>MAAQNEQRPERIKTTPYLEGDVLSSDSGPLLSVFALQEIMQKVRQVQADYMTATREVDFTVPDVQKILDDIKALAAEQVYKIVKVPSISFRHIVMQSRDRVLRVDTYYEEMSQVGDVITEDEPEKFYSTIIKKVRFIRGKGSFILHDIPTRDHRGMEVAEPEVLGVEFKNVLPVLTAEHRAMIQNALDGSIIENGNVATRDVDVFIGACSEPVYRIYNRLQGYIEAVQLQELRNSIGWLERLGHRKRITYSQEVLTDFRRQDTIWVLALQLPVNPQVVWDVPRSSIANLIMNIATCLPTGEYIAPNPRISSITLTQRITTTGPFAILTGSTPTAQQLNDVRKIYLALMFPGQIILDLKIDPGERMDPAVRMVAGVVGHLLFTAGGRFTNLTQNMARQLDIALNDYLLYMYNTRVQVNYGPTGEPLDFQIGRNQYDCNVFRADFATGTGYNGWATIDVEYREPAPYVHAQRYIRYCGIDSRELINPTTYGIGMTYHCYNEMLRMLVAAGKDSEAAYFRSMLPFHMVRFARINQIINEDLHSVFSLPDDMFNALLPDLIAGAHQNADPVVLDVSWISLWFAFNRSFEPTHRNEMLEVAPLIESVYASELSVMKVDMRHLSLMQRRFPDVLIQARPSHFWKAVLNDSPEAVKAVMNLSHSHNFINIRDMMRWVMLPSLQPSLKLALEEEAWAAANDFEDLMLTDQVYMHRDMLPEPRLDDIERFRQEGFYYTNMLEAPPEIDRVVQYTYEIARLQANMGQFRAALRRIMDDDDWVRFGGVLRTVRVKFYDARPPDDVLQGLPFSYDTNERGGLAYATIKYATETTIFYLIYNVEFSNTPDSLVLINPTYTMTKVFINKRIVERVRVGQILAVLNRRFVAYKGKMRIMDITQSLKMGTKLAAPTV[10x];>MSAAMLLAPGDVIKRSSEELKQRQIQINLIDWTEGESEKESKAEAKEGDKAEELKDGEGTQSESSQKKESSKETKDADVDRRIHTAVGSGSSAKGPGERANENVDRGDGKVGGGGGDADAGVGATGANGGRWVVLTEEIARAIESKYGTKIDVYRDEVPAQIIEVERSLQKELGISREGVAEQTERLRDLRRKEKSGAHAKA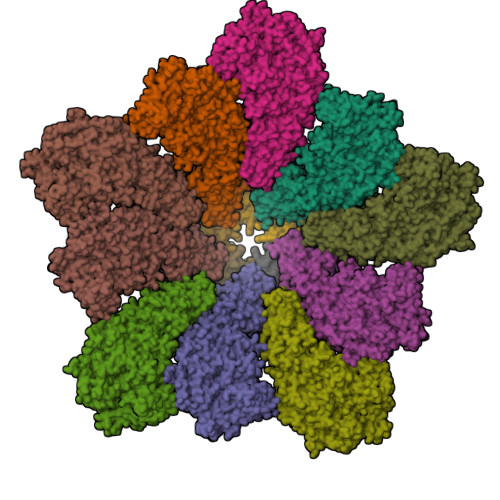AERGRRKQGKKPHGDAQREGTEEEKTSEEPASVGITIEGVMSQKKLLSMIGGVERKMAPIGARESAVMLVSNSIKDVVRATAYFTAPTGDPHWKEVAREASKKKNILAYTSTGGDVKTEFLHLIDHL[5x]> MVKSYQRFEQAAAFGVIASNANCVWIPASSGN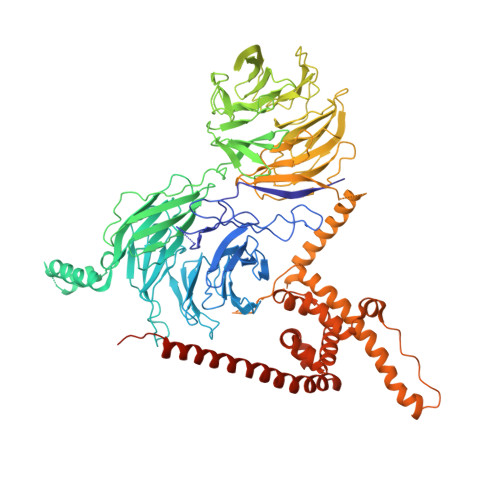SNGSGPGQLITSALEDVNIWDIKTGDLVSKLSDGLPPGASDARGAKPAECTYLEAHKDTDLLAVGYADGVIKVWDLMSKTVLLNFNGHKAAITLLQFDGTGTRLISGSKDSNIIVWDLVGEVGLYKLRSHKDSITGFWCQGEDWLISTSKDGMIKLWDLKTHQCIETHIAHTGECWGLAVKDDLLITTGTDSQVKIWKLDIENDKMGGKLTEMGIFEKQSKQRGLKIEFITNSSDKTSFFYIQNADKTIETFRIRKEEEIARGLKKREKRLKEXXXXXXXXXXYSSFILHPFQTIRSLYKIKSASWTTVSSSKLELVLTTSSNTIEYYSIPYEKRDPTSPAPLKTHTIELQGQRTDVRSIDISDDNKLLATASNGSLKIWNIKTHKCIRTFECGYALTCKFLPGGLLVILGTRNGELQLFDLASSSLLDTIEDAHDAAIWSLDLTSDGKRLVTGSADKTVKFWDFKVENSLVPGTKNKFLPVLKLHHDTTLELTDDILCVRVSPDDRYLAISLLDNTVKVFFLDSMKFYLSLYGHKLPVLSIDISFDSKMIITSSADKNIKIWGLDFGDCHKSLFAHQDSIMNVKFLPQSHNFFSCSKDAVVKYWDGEKFECIQKLYAHQSEVWALAVATDGGFVVSSSHDHSIRIWEETEDXXXXXXXXXXXXXXXXXXXXXXXXXSGVHKQTLESLKAGERLMEALDLGIAEIEGLEAYNRDMKLWQRKKLGEAPIKPQGNAVLIAVNKTPEQYIMDTLLRIRMSQLEDALMVMPFSYVLKFLKFIDTVMQNKTLLHSHLPLICKNLFFIIKFNHKELVSQKNEELKLQINRVKTELRSALKSTEDDLGFNVQGLKFVKQQWNLRHNYEFVDEYDQQEKESNSARKRVFGTVI>MEEKSKGNLVIIGGAEDKKGESKILKKVAEIAGFGDMEFIVLTTATEHPVEVGNEYLNVFQRLGINNIEVLDISTREDANNEENYYKIVNSGGVFMTGGDQLRIT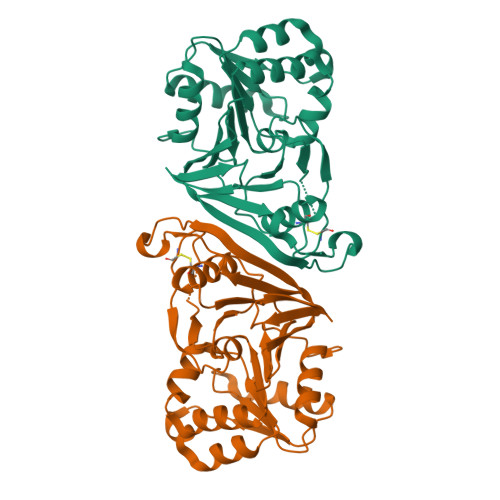SILGGTKVFNALIEAYLKGVVIAGTSAGASVMSNTMIVDGNSNDPARKCTLKMASGLGLLEEAIIDQHFDQRGRFGRLLCGVAENPHMLGIGIDEDTAIRVYPDAHFEVVGSYAVTIIDGKSIVSSNVSELKPDEILAIANVTVHVLPEGYGFDMKRREVLRLHENLYFQ[4x]> MVKFLGAVPVLTAVDVPANVSFWVDTLGFEKDFGDRDFA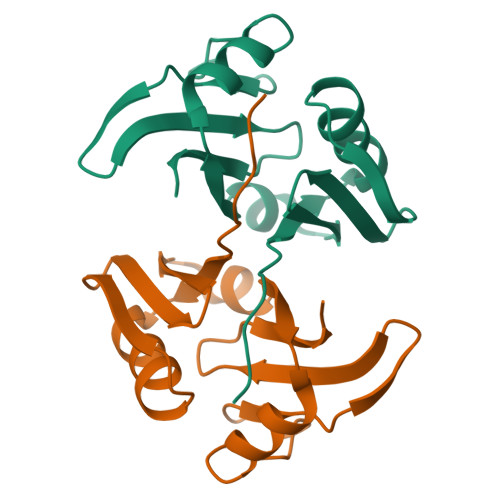GVRRGDIRLHISRTEHQIVADNTSAWIEVTDPDALHEEWARAVSTDYADTSGPAMTPVGESPAGREFAVRDPAGNCVHFTAGE>[2x]DILECDYFDTVDISAAQKLQNGSYLFEGLLVPAILTGEYDFRILPDDSKQKVARHIRGCVCKLKPCVRFCCPHDHIMDNGVCYDNMSDEELAELDPFL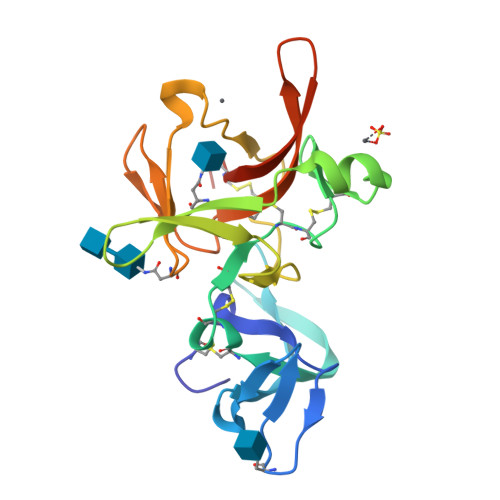NVTLDDGSVSRRHFKNELIVQWDLPMPCDGMFYLDNREEQDKYTLFENGTFFRHFDRVTLRKREYCLQHLTFADGNATSIRIAPHNCLIVPSITGQT> MQVNRLPFFTNHFFDTYLLISEDTPVGSSVTQLLARDMDNDPLVFGVPGEEASRFFAVEPDTGVVWLRQPLDRETKSEFTVEFSVSDHQGVITRKVNIQVGDVNDNAPTFHNQPYSVRIPENTPVGTPIFIVNATDPDLGAGGSVLYSFQPPSPFFAIDSARGIVTVIQELDYEVTQAYQLTVNATDQDKTRPLSTLANLAIIITDLEHHHHHH;> MQYDDDWQYEDCKLARGGPPATIVAIDEESRNGTILVDNMLIKGTAGGPDPTIELSLKDNVDYWVLLDPVKQMLFLNSTGRVLDRDPPMNIHSIVVQVQCVNKKVGTVIYHEVRIVVRDRNDNSPTFKHESYYATVNELTPVGTTIFTGFSGDNGATDIDDGPNGQIEYVIQYNPEDPTSNDTFEIPLMLTGNVVLRKRLNYEDKTRYYVIIQANDRAQNLNERRTTTT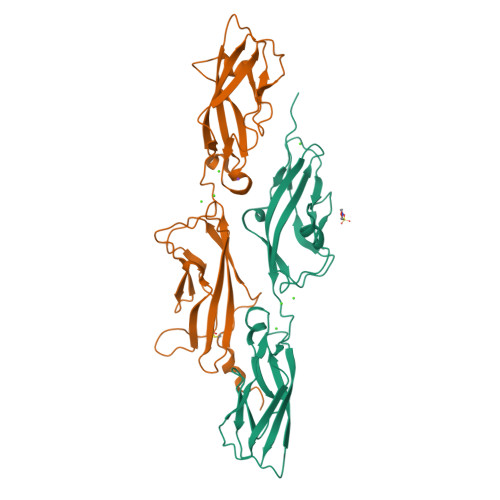TLTVDLEHHHHHH> YSIEADKKFKYSVKLSDYPTLQDAASAAVDGLLIDRDYNFYGGETVDFGGKVLTIECKAKFIGDGNLIFTKLGKGSRIAGVFMESTTTPWVIKPWTDDNQWLTDAAAVVATLKQSKTDGYQPTVSDYVKFPGIETLLPPNAKGQNITSTLEIRECIGVEVHRASGLMAGFLFRGCHFCKMVDANNPSGGKDGIITFENLSGDWGKGNYVIGGRTSYGSVSSIQFLRNNGGFERDGGVIGFTSYRAGESGVKTWQGTVGSTTSRNYNLQFRDSVVIYPVWDGFDLGADTDMNPELDRPGDYPITQYPLHQLPLNHLIDNLLVRGALGVGFGMDGKGMYVSNITVEDCAGSGAYLLTHESVFTNIAIIDTNTKDFQANQIYISGACRVNGLRLIGIRSTDGQGLTIDAPNSTVSGITGMVDPSRINVANLAEEGLGNIRANSFGYDSAAIKLRIHKLSKTLDSGALYSHINGGAGSGSAYTQLTAISGSTPDAVSLKVNHKDCRGAEIPFVPDIASDDFIKDSSCFLPYWENNSTSLKALVKKPNG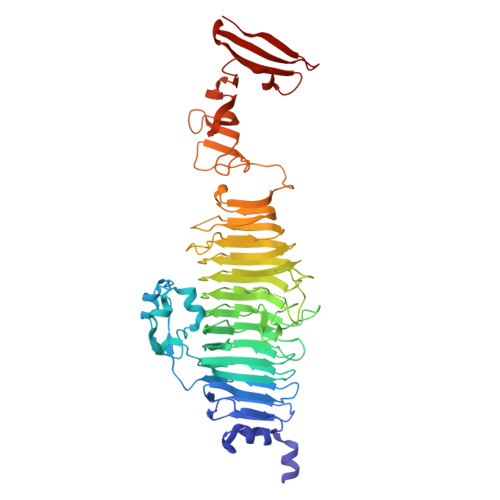ELVRLTLATL> GTSQVINGEMQFYARAKLFYQEVPATEEGMMGNFIELSSPDIQASQKFLRKFVGGPGRAGTDCALDCGSGIGRVSKHVLLPVFNSVELVDMMESFLLEAQNYLQVKGDKVESYHCYSLQEFTPPFRRYDVIWIQWVSG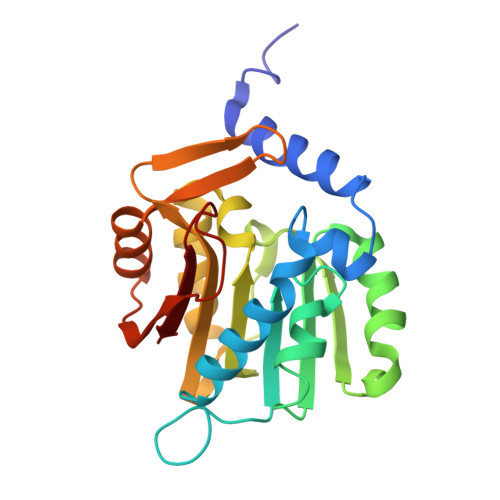HLTDKDLLAFLSRCRDGLKENGIIILKDNVAREGCILDLSDSSVTRDMDILRSLIRKSGLVVLGQEKQDGFPEQCIPVWMFALH> MGSSHHHHHHTNKYHEKWISKFAPGNELSKKYLAK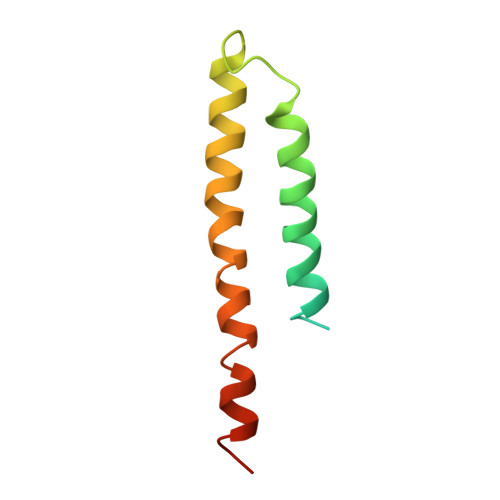VKERHELKEFNNSISAQDNYAKWTKNNRKLDSLDKEINNLKDEIQSENKAFQAHLHKLR>[2x]HMDEQIPHDKSLDNSLTLLKEGYLFIKNRTERYNSDLFQARLLGKNFICMTGAEAAKVFYDTDRF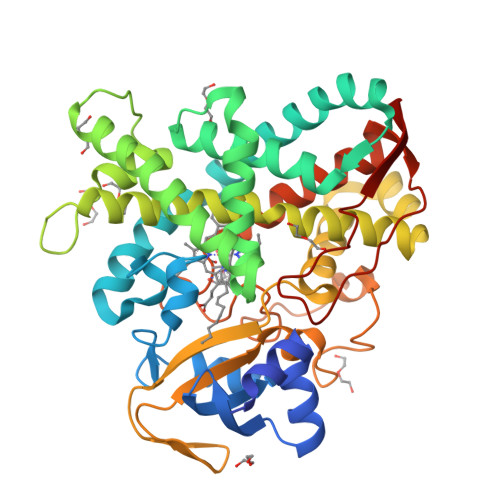QRQNALPKRVQKSIFGVNAIHGMDGSAHIHRKMLFLSLMTPPHQKRLAELMTEEWKAAVTRWEKADEVVLFEEAKEILCRVACYWAGVPLKETEVKERADDFIDMVDAFGAVGPRHWKGRRARPRAEEWIEVMIEDARAGLLKTTSGTALHEMAFHTQEDGSQLDSRMAAIELINVLRPIVAISYFLVFSALALHEHPKYKEWLRSGNSREREMFVQEVRRYYPFIPFLGALVKKDFVWNNCEFKKGTSVLLDLYGTNHDPRLWDHPDEFRPERFAEREENLFDMIPQGGGHAEKGHRCPGEGITIEVMKASLDFLVHQIEYDVPEQSLHYSLARMPSLPESGFVMSGIRRKS>MSVEVSRGLENVIIKTTGLTYIDGINGILRYRGYDINDLVNYASYEELIHLMLYGELPNRQQLNQIKGIINESFEVPEQVISTIFSMPRNCDAIGMMETAFGILASIYDPKWNRATNKELAVQIIAKTATITANIYRAKEGLKPKIPEPSESYAESFLAATFGKKPTQEEIKAMDASLILYTDHEVPASTTAALVASSTLSDMYSCIVAALAALKGPLHGGAAEEAFKQFVEIGSVENADKWFEEKIIKGKSRLMGFGHRVYKTYDPRAKIFKTLAKSFAE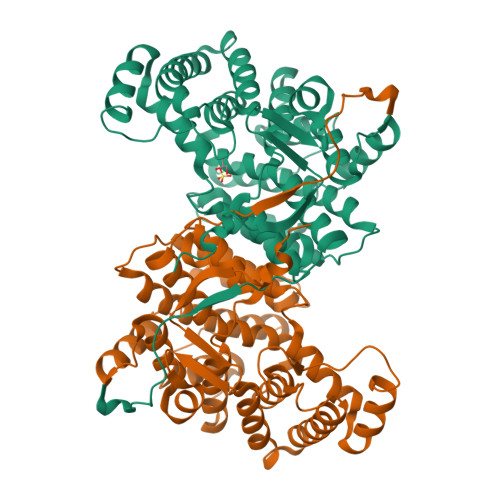KNENVKKYYEIAERIEKLGVDTFGSKHIYPNTDFYSGIVFYALGFPIYMFTSLFALSRVLGWLAHIIEYVEEQHRLIRPRALYIGPEKREFKPIELR[2x]>[4x]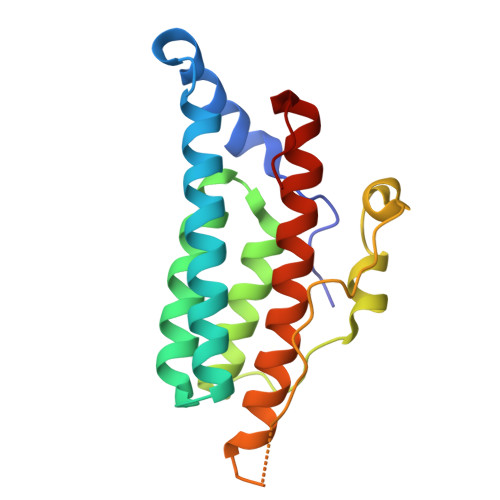MSTIPSEIINWTILNEIISMDDDDSDFSKGLIIQFIDQAQTTFAQMQRQLDGEKNLTELDNLGHFLKGSSAALGLQRIAWVCERIQNLGRKMEHFFPNKTELVNTLSDKSIINGINIDEDDEEIKIQVDDKDENSIYLILIAKALNQSRLEFKLARIELSKYYNTNLH> SSAVAILETFQKYTIDQKKDTAVRGLARIVQVGENKTLFDITVNGVPEAGNYHASIHEKGDVSKGVESTGKVWHKFDEPIE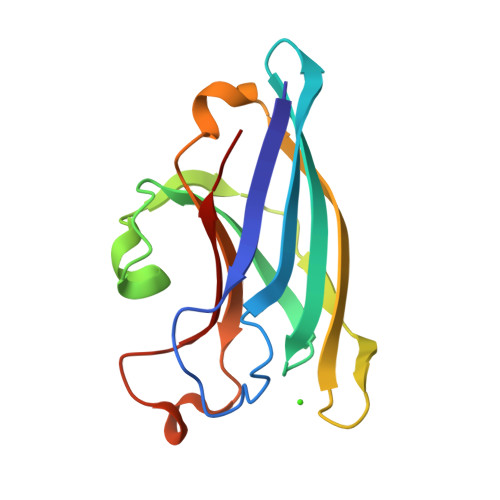CFNESDLGKNLYSGKTFLSAPLPTWQLIGRSFVISKSLNHPENEPSSVKDYSFLGVIAR Indanomycin is an antibiotic from the pyrroloketo­indane family which is known to act as an effective ionophoric agent against Gram-positive bacteria. IdmH is a homodimer, with the individual protomers consisting of an α+β barrel. Each protomer contains a deep hydrophobic pocket which is proposed to constitute the active site of the enzyme.

X-ray diffraction data were collected to 2.7 Å resolution, but attempts to determine the structure by molecular replacement were unsuccessful, presumably owing to the lack of a suitable search model and the large number of molecules in the asymmetric unit as estimated using MATTPROB. The remainder of the structural description will focus on the unlabelled native protein as this should best represent the natural form of the enzyme. With this structure in hand, the crystal structure of wild-type IdmH was determined by molecular replacement using a single subunit of IdmH-Δ99–107 as a search model. Electron-density maps were well defined for all ten protomers in the asymmetric unit, allowing all chains to be modelled, with the exception of some residues at the extreme N- and C-termini (residues in the ranges 1–6 and 143–148). The ten molecules in the asymmetric unit for the wild-type protein form five almost identical dimers. The following discussion of the IdmH structure will therefore focus on the dimer formed by chains A and B unless otherwise stated, as this represents the most well ordered dimer based on an analysis of the overall B factors of the chains. Two loops (residues 38–46 and 99–108) are located near to the entrance of this hydrophobic pocket and limit the access to the proposed active site from the bulk solvent. Interestingly, the loop, which comprises residues 99–108 and is partially truncated in the IdmH-Δ99–107 variant, appears to occupy two distinct conformations within each of the five dimers in the asymmetric unit. Indeed, in each dimer each protomer has this loop occupying either a more open or a more closed conformation above the hydrophobic cavity. Whilst we cannot rule this out as an artefact of the crystallization, this suggests that this loop is likely to be highly dynamic in solution and may also hint at a potential change in conformation between the two protomers, suggesting the potential for allostery in this enzyme. Indanomycin was placed in the wild-type IdmH active sites (chain A and B) using in silico molecular docking.

>[10x]GSHMAHQPSDTIAGLYEAFNSGDLETLRELIAPDAVIHLPGTAGDAEHPPGTPRDREGWLGVWQFTQAFFPDMTATVQDIVQTGDLVATRCVARGTHSIEFMGVPPTGRPFEMTMLNMSRVRDGRIVEHWTISDNVTMLAQLGVKASL> MSQSNRELVVDFLSYKLSQKGYSWSQMAAVKQALREAGDEFELRYRRAFSDLTSQLHITPGTAYQSFEQVVNELFRDG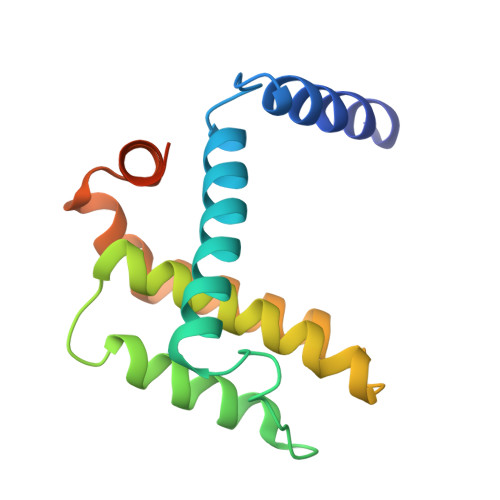VNWGRIVAFFSFGGALCVESVDKEMQVLVSRIAAWMATYLNDHLEPWIQENGGWDTFVELYGNNAAAESRKGQER> NREEKILNREIGFAIGMPVCEFDMVKDPEVQDFRRNILNVCKEAVDLRDLNSPHSRAMYVYPPNVESSPELPKHIYNKLDKGQIIVVIWVIVSPNNDKQKYTLKINHDCVPEQVIAEAIRKKTRSMLLSSEQLKLCVLEYQGKYILKVCGCDEYFLEKYPLSQYKYIRSCIMLGRMPNLMLMAKESLYSQLPMDCFTMPSYSRRISTATPYMNGETSTKSLWVINSALRIKILCATYVNVNIRDIDKIYVRTGIYHGGEPLCDNVNTQRVPCSNPRWNEWLNYDIYIPDLPRAARLCLSICSVKGRKGAKEEHCPLAWGNINLFDYTDTLVSGKMALNLWPVPHGLEDLLNPIGVTGSNPNKETPCLELEFDWFSSVVKFPDMSVIEEHANWSVSREAGFSYSHAGLSNRLARDNELRENDKEQLKAISTRDPLSEITEQEKDFLWSHRHYCVTIPEILPKLLLSVKWNSRDEVAQMYCLVKDWPPIKPEQAMEL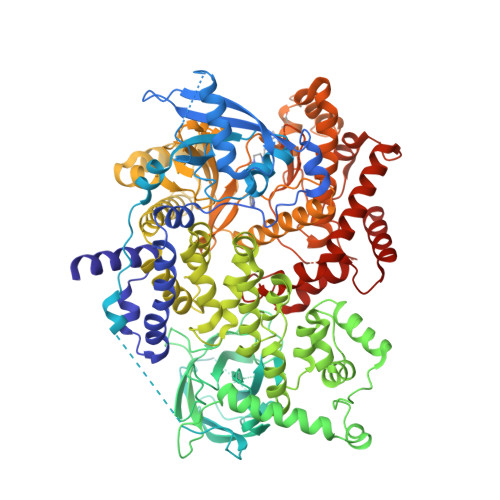LDCNYPDPMVRGFAVRCLEKYLTDDKLSQYLIQLVQVLKYEQYLDNLLVRFLLKKALTNQRIGHFFFWHLKSEMHNKTVSQRFGLLLESYCRACGMYLKHLNRQVEAMEKLINLTDILKQEKKDETQKVQMKFLVEQMRRPDFMDALQGFLSPLNPAHQLGNLRLEECRIMSSAKRPLWLNWENPDIMSELLFQNNEIIFKNGDDLRQDMLTLQIIRIMENIWQNQGLDLRMLPYGCLSIGDCVGLIEVVRNSHTIMQIQCKGGLKGALQFNSHTLHQWLKDKNKGEIYDAAIDLFTRSCAGYCVATFILGIGDRHNSNIMVKDDGQLFHIDFGHFLDHKKKKFGYKRERVPFVLTQDFLIVISKGAQECTKTREFERFQEMCYKAYLAIRQHANLFINLFSMMLGSGMPELQSFDDIAYIRKTLALDKTEQEALEYFMKQMNDA> QQNVWPRTFQNADGSITTIPSQPKRILSTAVTVTGTLLAIDAPVIASAATTQSTFFEQWRKLAELRQVKKLWPAGSVDLESVYVEQPDLIVVSMIGADSARDQIPLLQAIAPTILVDYSDQTWQSLAQQLGLATGLEEQAERTIHNFEQWTKQVRDVLDLPKGRANIVSYHGPGVVNAVAKAQSAHAQLLQSVGVVLEEPDPAWQAGSIVHRDFLRIHYEHLTQLQAETTFLIT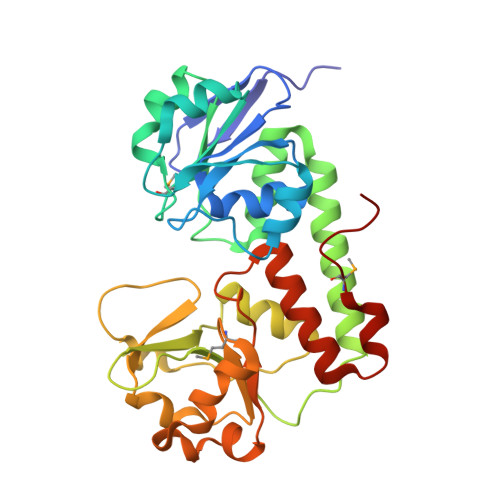MTDQQAQAFLHDPILKNLPSIQRKQVYGLGENSFRIDLFSAREIINSLLRRFAGEQAQSLVMPLEHHHHHH>MDVNVRGPDGFTPLMIASCSGGGLETGNSEEEEDAPAVISDFIYQGASLHNQTDRTGETALHLAARYSRSDAAKRLLEASADANIQDNMGRTPLHAAVSADAQGVFQILIRNRATDLDARMHDGT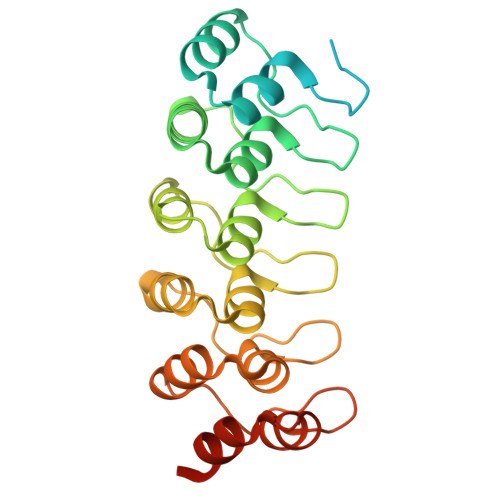TPLILAARLAVEGMLEDLINSHADVNAVDDLGKSALHWAAAVNNVDAAVVLLKNGANKDMQNNREETPLFLAAREGSYETAKVLLDHFANRDITDHMDRLPRDIAQERMHHDIVRLLDLEHHHHHHHH[2x]> GPISPIETVPVKLKPGMDGPKVKQWPLTEEKIKALVEICTEMEKEGKISKIGPENPYNTPVFAIKKKDGTKWRKLVDFRELNKKTQDFWEVQLGIPHPAGLKKKKSVTVLDVGDAYFSVPLDEDFRKYT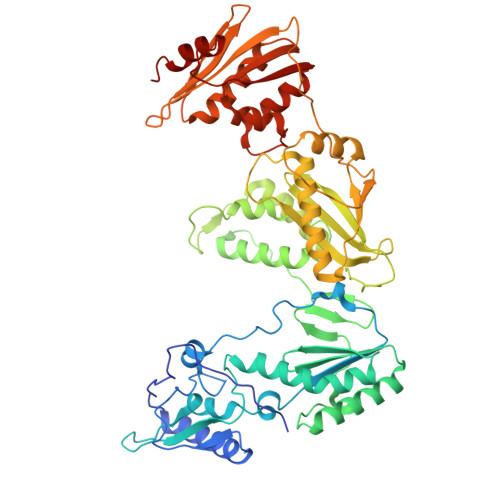AFTIPSINNETPGIRYQYNVLPQGWKGSPAIFQSSMTKILEPFRKQNPDIVIYQYMDDLYVGSDLEIGQHRTKIEELRQHLLRWGLTTPDKKHQKEPPFLWMGYELHPDKWTVQPIVLPEKDSWTVNDIQKLVGKLNWASQIYPGIKVRQLCKLLRGTKALTEVIPLTEEAELELAENREILKEPVHGVYYDPSKDLIAEIQKQGQGQWTYQIYQEPFKNLKTGKYARMRGAHTNDVKQLTEAVQKITTESIVIWGKTPKFKLPIQKETWETWWTEYWQATWVPEWEFVNTPPLVKLWYQLEKEPIVGAETFYVDGAASRETKLGKAGYVTNKGRQKVVTLTDTTNQKTELQAIHLALQDSGLEVNIVTDSQYALGIIQAQPDQSESELVNQIIEQLIKKEKVYLAWVPAHKGIGGNEQVDKLVSAGIR>MKTPLVTREGYEKLKQELNYLWREERPEVTKKVTWAASLGDRSENADYQYNKKRLREIDRRVRYLTKCMENLKIVDYSPQQEGKVFFGAW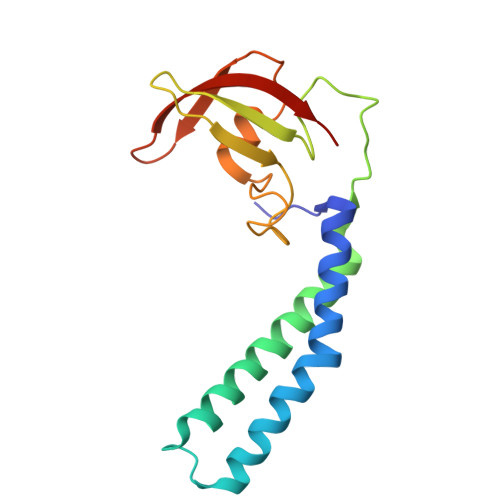VEIENDDGVTHRFRIVGYDEIFGRKDYISIDSPMARALLKKEVGDLAVVNTPAGEASWYVNAIEYVKP[6x]>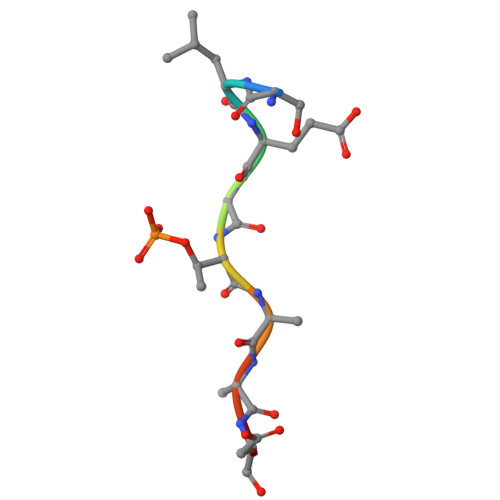 SLEVTEADT> GSYDRNHTYIVSSLLEEPYLSLKQYTYGESLVGNDRFEGYCKDLADMLAAQLGIKYEIRLVQDGNYGAENQYAPGGWDGMVGELIRKEADIAISAMTITAERERVIDFSKPFMT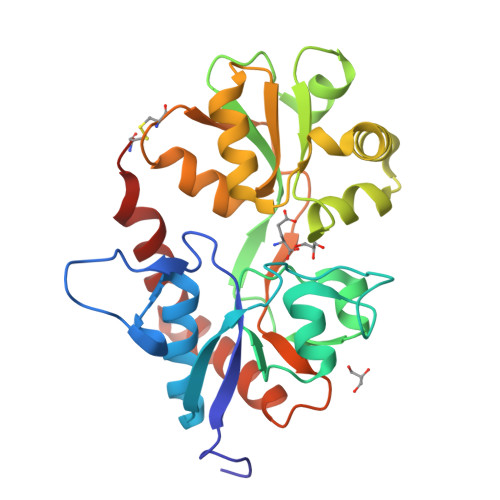LGISIMIKKGTPIKTPEDLTMQTDVNYGTLLYGSTWEFFRRSQIGLHNKMWEYMNANQHHSVHTTDEGIRRVRQSKGKYALLVESPKNEYVNARPPCDTMKVGRNIDTKGFGVATPIGSPLRKRLNEAVLTLKENGELLRIRNKWWFDKTECN> MEFVAKLFKFFKDLLGKFLGN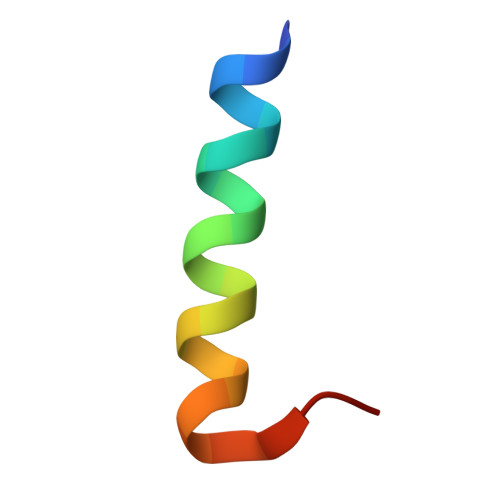NX>[2x]MDYKDDDDKGSSSSNVEVFIPVSQGNTNGFPATASNDLKAFTEGAVLSFHNICYRVKLKSGFLPCRKPVEKEILSNINGIMKPGLNAILGPTGGGKSSLLDVLAARKDPSGLSGDVLINGAPRPANFKCNSGYVVQDDVVMGTLTVRENLQFSAALRLATTMTNHEKNERINRVIQELGLDKVADSKVGTQFIRGVSGGERKRTSIGMELITDPSILFLDEPTTGLDSSTANAVLLLLKRMSKQGRTIIFSIHQPRYSIFKLFDSLTLLASGRLMFHGPAQEALGYFESAGYHCEAYNNPADFFLDIINGDSTAVALNREEDFKATEIIEPSKQDKPLIEKLAEIYVNSSFYKETKAELHQLSGGEKKKKITVFKEISYTTSFCHQLRWVSKRSFKNLLGNPQASIAQIIVTVVLGLVIGAIYFGLKNDSTGIQNRAGVLFFLTTNQCFSSVSAVELFVVEKKLFIHEYISGYYRVSSYFLGKLLSDLLPMRMLPSIIFTCIVYFMLGLKPKADAFFVMMFTLMMVAYSASSMALAIAAGQSVVSVATLLMTICFVFMMIFSGLLVNLTTIASWLSWLQYFSIPRYGFTALQHNEFLGQNFCPGLNATGNNPCNYATCTGEEYLVKQGIDLSPWGLWKNHVALACMIVIFLTIAYLKLLFLKKYS

ABCG2 is an ABC transporter of broad substrate specificity expressed in various tissues and tissue barriers. ABCG2 also functions as a multidrug transporter and exports a wide range of xenobiotics and pharmaceuticals, thus strongly impacting their pharmacokinetics. Here we present cryo-EM structures of ABCG2 under turnover conditions containing either the endogenous substrate estrone-3-sulfate or the exogenous substrate topotecan. We find two distinct conformational states in which both the transport substrates and ATP are bound.

The turnover sample containing E1S revealed a single, well-defined conformation resolved at 3.4 Å resolution. The conformation of the E1S-bound structure was very similar to turnover-2 from the topotecan-containing sample. We, therefore, refer to the E1S-bound structure as turnover-2 as well. In the structure containing E1S (turnover-2), the substrates could be fit in two orientations related approximately by a 180° rotation. When compared to the previously reported structure of E1S- and 5D3-Fab-bound ABCG2 in an inward-open conformation, E1S appeared slightly shifted (~1 Å) towards the leucine gate and thus towards the external side of the transporter. In the topotecan-bound ABCG2 sample, the dominant class (88% of the ordered particles) belonged to the turnover-1 state, whereas 12% particles belonged to the turnover-2 state. This suggests that turnover-1 is the lowest-energy state of ABCG2 in the presence of topotecan, whereas turnover-2 is the lowest-energy state in the presence of E1S. Given that E1S did not promote the turnover-1 state, we concluded that ABCG2 can directly proceed to turnover-2 when smaller or endogenous substrates are bound. For these substrates, turnover-2 appears to immediately precede the rate-limiting step of the transport cycle. In contrast, the strongly reduced size of cavity 1 in the turnover-2 conformation would lead to major steric clashes with bound inhibitor molecules. Figure 5 reveals that whereas there is sufficient space in turnover-2 for bound substrates (E1S or topotecan), the inhibitors MZ29 and MB136 could not fit.>STYADYFSAWDKWEKQALPGEERDEAVSRLKECLINNSDELRLDRLNLSSLPDNLPAQITLLNVSYNQLTNLPELPVTLKKLYSASNKLSELPVLPPALESLQVQHNELENLPALPDSLLTMNISYNEIV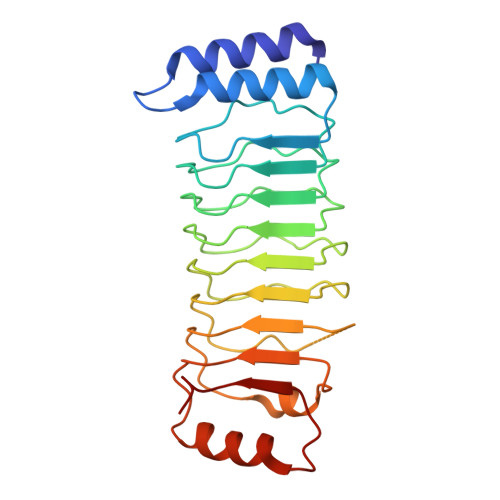SLPSLPQALKNLRATRNFLTELPAFSEGNNPVVREYFFDRNQISHIPESILNLRNECSIHISDNPLSSHALPALQRLTSSPDYHGPRIYFSMSD[2x]>[2x]SIIRPQLKFREKIDNSNTPFLPKIFIKPNAQKPLPQALSKERRERPQDRPEDLDVPPALADFIHQQRTQQVEQDMFAHPYQYELNHFTPADAVLQKPQPQLYRPIEETPCHFISSLDELVELNEKLLNC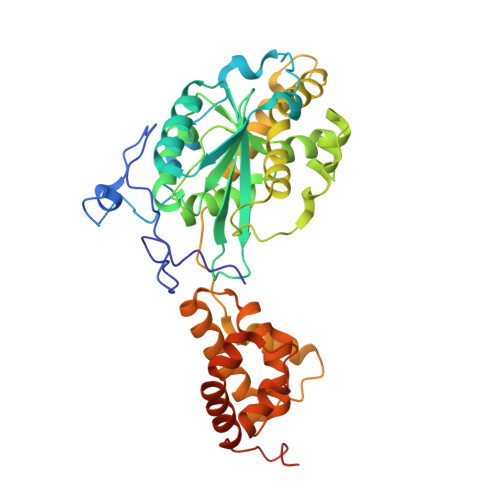QEFAVDLEHHSYRSFLGLTCLMQISTRTEDFIIDTLELRSDMYILNESLTDPAIVKVFHGADSDIEWLQKDFGLYVVNMFDTHQAARLLNLGRHSLDHLLKLYCNVDSNKQYQLADWRIRPLPEEMLSAARDDTHYLLYIYDKMRLEMWERGNGQPVQLQVVWQRSRDICLKKFIKPIFTDESYLELYRKQKKHLNTQQLTAFQLLFAWRDKTARREDESYGYVLPNHMMLKIAEELPKEPQGIIACCNPVPPLVRQQINEMHLLIQQAREMPLLKSEVAAGVKKSGPLPSAERLENVL> MSGSLREEIRKLAEQLSEKYKDEEIRELAREAAELAEESDDPEVLELAYEALKKGLELEDEEKVKLILLAAVLAARVARGEVPEEKLEIALKALELAEASEDERIIRGALRAALAAARTDDPLALEVVLEALERAQASEDERLIRAILAAAYAFALLAVAGASAERLKEAEAIVKELIAAAEKGASPQELVLLVIEMMVKGMGVTMETHRSGNEVKVVIKGLHESQQEVLLEAVLFAAELMGVR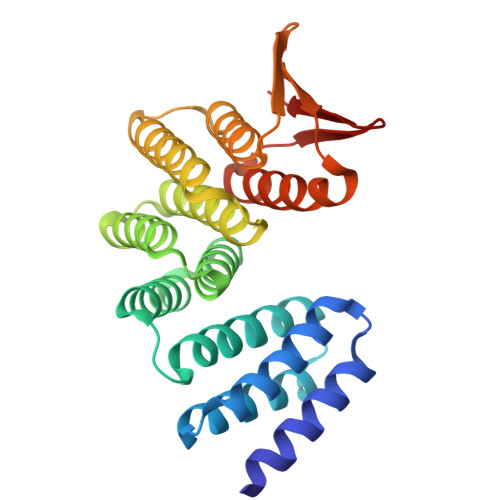VRIRFKGDTVTIVVRE>[2x]MSNTKTASTGFAELLKDRREQVKMDHAALASLLGETPETVAAWENGEGGELTLTQLGRIAHVLGTSIGALTPPAGNDLDDGVIIQMPDERPILKGVRD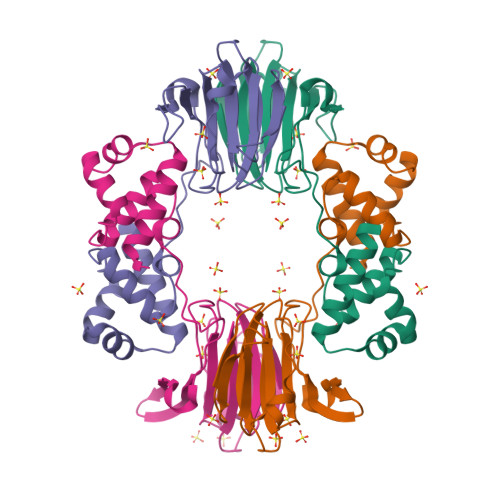NVDYYVYNCLVRTKRAPSLVPLVVDVLTDNPDDAKFNSGHAGNEFLFVLEGEIHMKWGDKENPKEALLPTGASMFVEEHVPHAFTAAKGTGSAKLIAVNF> AQTPAFDKPKVELHVHLDGAIKPETILYYGKRRGIALPADTPEELQNIIGMDKPLT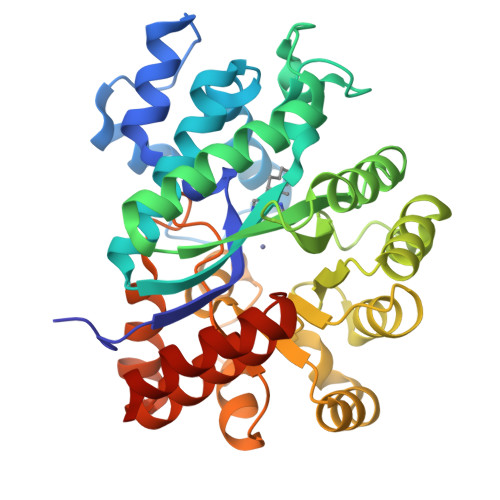LPDFLAKFDYYMPAIAGCRDAIKRIAYEFVEMKAKDGVVYVEVRYSPHLLANSKVEPIPWNQAEGDLTPDEVVSLVNQGLQEGERDFGVKVRSILCCMRHQPSWSSEVVELCKKYREQTVVAIDLAGDETIEGSSLFPGHVQAYAEAVKSGVHRTVHAGEVGSANVVKEAVDTLKTERLGHGYHTLEDTTLYNRLRQENMHFEICPWSSYLTGAWKPDTEHAVIRFKNDQVNYSLNTDDPLIFKSTLDTDYQMTKKDMGFTEEEFKRLNINAAKSSFLPEDEKKELLDLLYKAYRMPSPA>PANLLTSLVRAHLDSGPSTAKLDYSKFQELVLPHFGKEDAGDVQQFYDLLSGSLEVIRKWAEKIPGFAELSPADQDLLLESAFLELFILRLAYRSKPGEGKLIFCSGLVLHRLQCARGFGDWIDSILAFSRSLHSLLVDVPAFACLSALVLITDRHGLQEP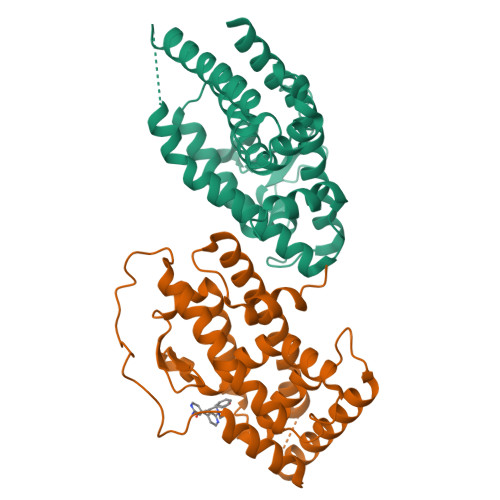RRVEELQNRIASCLKEHVAAVAGEPQPASCLSRLLGKLPELRTLCTQGLQRIFYLKLEDLVPPPPIIDKIFMDTLPF[2x]> AQVLRGTVTDFPGFDERADAETLRKAMKGLGTDEESILTLLTSRSNAQRQEISAAFKTLFGRDLLDDLKSELTGKFQKLIVALMKPSRLYDAYELKHALKGAGTNEKVLTEIIASRTPEELRAIKQVYEEEYGSSLEDDVVGDTSGYYQRMLVVLLQANRDPDAGIDEAQVEQDAQALFQAGELKWGTDEEKFITIFGTRSVSHLRKVFDKYMTISGFQIEETIDRETSG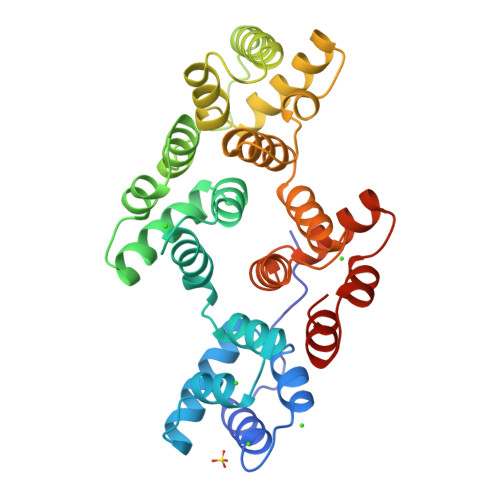NLEQLLLAVVKSIRSIPAYLAETLYYAMKGAGTDDHTLIRVMVSRSEIDLFNIRKEFRKNFATSLYSMIKGDTSGDYKKALLLLCGEDD>[2x]AVSKVYARSVYDSRGNPTVEVELTTEKGVFRSIVPSGASTGVHEALEMRDGDKSKWMGKGVLHAVKNVNDVIAPAFVKANIDVKDQKAVDDFLISLDGTANKSKLGANAILGVSLAASRA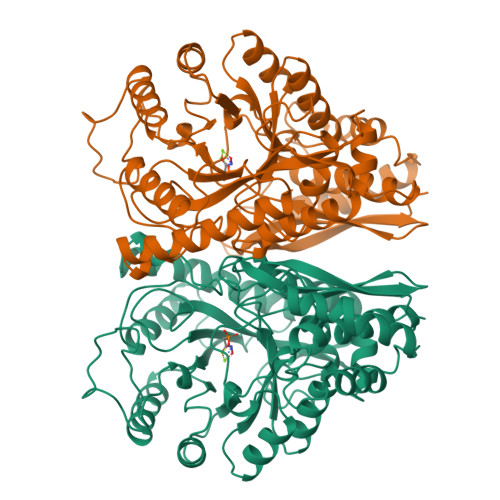AAAEKNVPLYKHLADLSKSKTSPYVLPVPFLNVLNGGSHAGGALALQEFMIAPTGAKTFAEALRIGSEVYHNLKSLTKKRYGASAGNVGDEGGVAPNIQTAEEALDLIVDAIKAAGHDGKVKIGLDCASSEFFKDGKYDLDFKNPNSDKSKWLTGPQLADLYHSLMKRYPIVSIEDPFAEDDWEAWSHFFKTAGIQIVADDLTVTNPKRIATAIEKKAADALLLKVNQIGTLSESIKAAQDSFAAGWGVMVSHRSGETEDTFIADLVVGLRTGQIKTGAPARSERLAKLNQLLRIEEELGDNAVFAGENFHHGDKL>GPGPEYQAQGLAMYLQENGIDCPKCKFSYALARGGCMHFHCTQCRHQFCSGCYNAFYAKNKCPEPNCRVKKSLHGHHPRDCLFYLRDWTALRLQKLLQDNNVMFNTEPPAGARAVPGGGCRVIEQKEVPNGLRDEACGKETPAG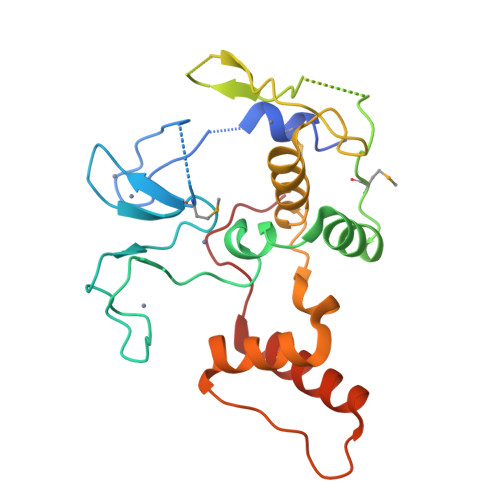YAGLCQAHYKEYLVSLINAHSLDPATLYEVEELETATERYLHVRPQPLAGEDPPAYQARLLQKLTEEVPLGQSIPRRRK[4x]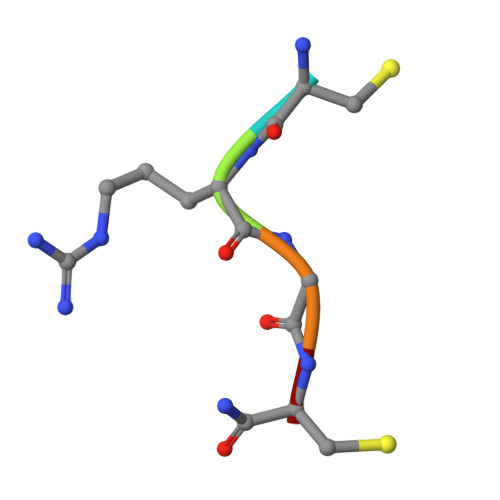> CRGCX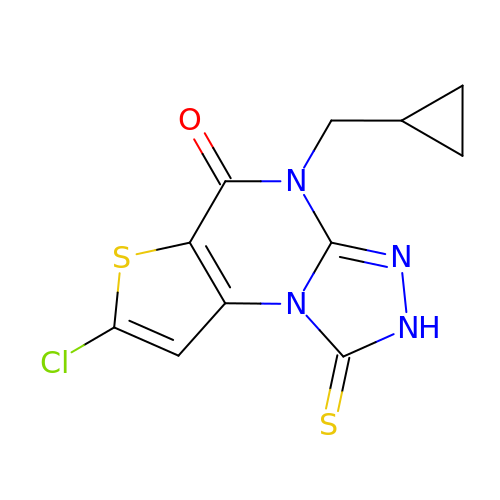7-chloro-4-(cyclopropylmethyl)-1-thioxo-2,4-dihydrothieno[2,3-e][1,2,4]triazolo[4,3-a]pyrimidin-5(1H)-one | C11 H9 Cl N4 O S2 | ACSIYLGZFSSIBQ-UHFFFAOYSA-N> MHEYAFFLGCIAPNRYPGCEASAIKTSEKVGIKLLPLKGASCCPAPGAFGSIDLNVWYAMAARNLVLAEEMKKDIALICNGCYKSIWEVNHILKHNDELRDNVNEVLAEIDMQFKGTI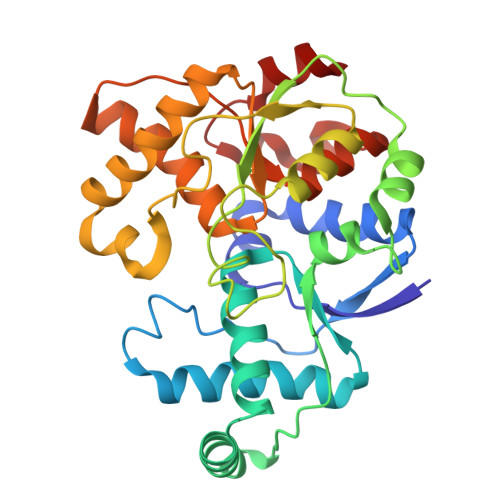DVWHLAELYYDDKVCGVQKIKDSVTTPLSGAKVAAHYGCHLMKPKKERHFGDTENPMWFEELIGALGAEPIQYRNKMQCCGAGGGVRGYDIVHALDITNEKLINIQEAGADAITELCPFCQLQFDRGQIEIKEKFGDVYNIPVLHYNELLGLAQGMSPQDLALDLHAIDCTPFLQKVL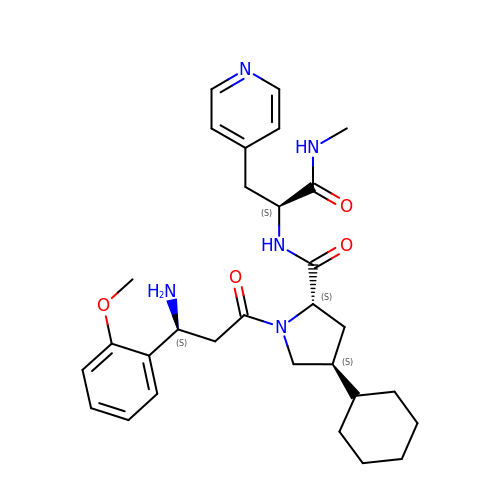(2~{S},4~{S})-1-[(3~{S})-3-azanyl-3-(2-methoxyphenyl)propanoyl]-4-cyclohexyl-~{N}-[(2~{S})-1-(methylamino)-1-oxidanylidene-3-pyridin-4-yl-propan-2-yl]pyrrolidine-2-carboxamide | C30 H41 N5 O4 | ZDWZDLUIZUBTKV-DNZIZEQUSA-N> SRENVPKSGTPQLRLPFAARLNTPMGPGRTVVVKGEVNANAKSFNVDLLAGKSKDIALHLNPRLNIKAFVRNSFLQESWGEEERNITSFPFSPGMYFEMIIYCDVREFKVAVNGVHSL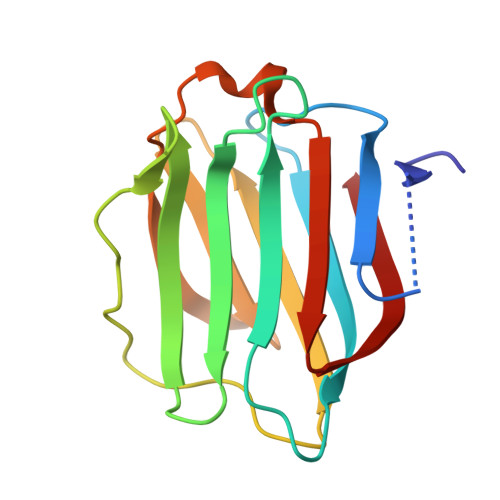EYKHRFKELSSIDTLEINGDIHLLEVRSW3-[[8-(1-methylindol-6-yl)quinoxalin-6-yl]amino]-~{N}-pyrimidin-5-yl-pyridine-4-carboxamide 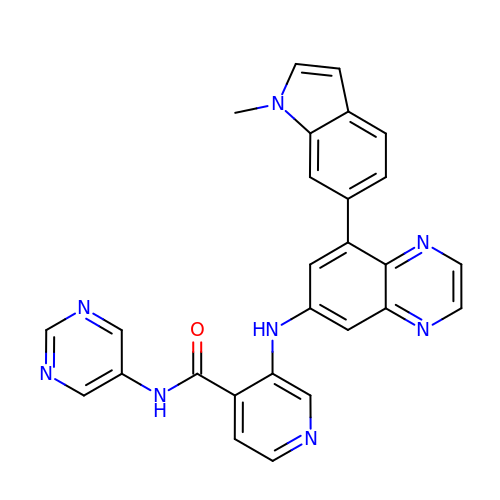| C27 H20 N8 O | VODZTUQHGMHXRJ-UHFFFAOYSA-N>MATLQDIGVSAGINILSAFVFFIIFAVLRLQPFNDRVYFSKWYLKGLRSSPARGGAFAQRFVNLDFRSYMKFLNWMPEALKMPEPELIDHAGLDSVVYLRIYWLGLKIFTPIAVLAWAVLVPVNWTNNTLEMAKQLRNVTSSDIDKLSVSNIPEYSMRFWTHIVMAYAFTIWTCYVLMKEYETIANMRLQFVASEARRPDQFTVLVRNVPPDADESVSELVEHFFLVNHPDHYLTHQVVCNANKLADLVKKKKKLQNWLDYYQLKYARNNSQRIMVKLGFLGLWGQKVDAIEHYIAEIDKISKEISKEREEVVNDPKAIMPAAFVSFKTRWAAAVCAQTQQTRNPTQWLTEWAPEPRDVFWSNLAIPYVSLTVRRLIMHVAFFFLTFFFIVPIAFVQSLATIEGIVKAAPFLKFIVDDKFMKSVIQGFLPGIALKLFLAFLPSILMIMSKFEGFTSISSLERRAAFRYYIFNLVNVFLASVIAGAAFEQLNSFLNQSANQIPKTIGVAIPMKATFFITYIMVDGWAGVAGEILMLKPLIMFHLKNAFLVKTDKDREEAMDPGSIGFNTGEPRIQLYFLLGLVYAPVTPMLLPFILVFFALAYIVYRHQIINVYNQEYESAAAFWPDVHGRVIAALVISQLLLMGLLGTKHAALAAPFLIALPVLTIGFHHFCKGRYEPAFIRYPLQEAMMKDTLETAREPNLNLKGYLQNAYVHPVFKGDEDDYDIDDKLGKFED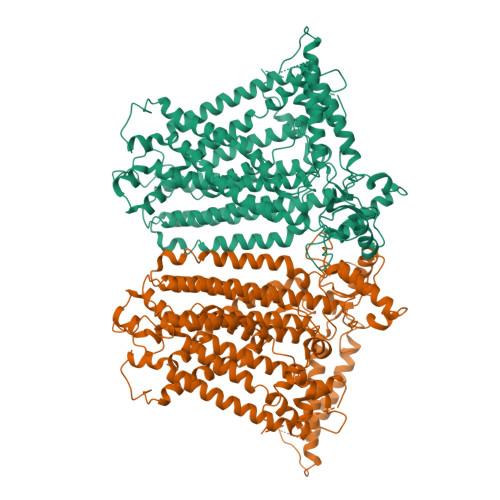EAIIVPTKRQSRRNTPAPSIISGDDSPSLPFSGKLV[2x]> MAEVVNGKLHLRFAIAPMRPTPSQTIKEFEPIFKYLADQLGATYEIVSPESWAAISVAMTNGHVDVGWLGPWGYVLSNKKAGTEVLATVKYRGEPFYKALIVGRADLPIKKWPEDAKGLKLSLSDQGNTSGWLIPMAYFKSIGIDPASYFEYREGATFGQNESQIQHGLIDLGSDMDRGRNGMIEAGQIDPSKSKIVWESSKLPNNAISVPKDFDPALKARITEILTSLSEEKAQSLMGSGYNGFVKAKHSDYKVIEDAGRILGKLLEHHHHHH

P. stutzeri WM88 has PtxABC, HtxBCDE and PhnCDE ABC-transporters for the acquisition of phosphite, hypophosphite and organophosphonates, respectively. These transport systems rely on a high-affinity periplasmic binding protein (PBP) to impart ligand specificity. HtxB is a typical type-II PBP, with a binding pocket positioned in a deep groove between two domains separated by a hinge region. A comparison of the HtxB and PtxB structures showed that sequence differences within the binding pocket essentially eliminate an oxygen binding site in HtxB, providing specificity for a ligand with two oxygen atoms (hypophosphite), over one with three (phosphite).

To probe the role of the D206 in ligand binding we generated D206A and D206N mutants of HtxB. The D206N mutation renders D206N HtxB incapable of binding phosphite or hypophosphite at pH 5 or 7.4, as determined by MST with up to 100 mM of ligand. Superposition of the ligand binding domain (residues 95–204) from D206N HtxB with WT HtxB shows that N206 points away from the ligand binding site in the mutant protein, rotated ca. 180° away from its position in the closed WT complex, and therefore, not in a position where it can interact with R178. We note that residue 206 sits on one of the two hinge regions of the protein (F96-K98 and P204-N206), suggesting it may have some flexibility. In the D206N HtxB structure, the sidechain oxygen of N206 sits within hydrogen bonding distance of the V89 amide (2.9 Å), altering the mainchain bond angles and rotating the N206 carbonyl by 50° away from its position in the WT/D206A HtxB structures. This change in mainchain conformation results in a 180° flip in the N205 carbonyl, requiring N205 to adopt a different rotamer in the D206N structure and leading to a new hydrogen bond formed with R178. It seems likely that this rearrangement of the mainchain very close to the hinge region, together with the concomitant change in the hydrogen bond network across the domain interface might result in the D206N HtxB mutant being unable to form a closed conformation in complex with phosphorus ligands, explaining why no ligand binding could be detected for this mutant in our solution studies. Comparisons of the D206N structure, which crystallised in a partially open conformation, with open and closed complexes from closely related proteins suggests that D206 and R178 are positioned on flexible regions of the protein that are brought into close proximity during domain closure.~{N}-[(2~{R},3~{R},4~{R},5~{S},6~{R})-5-[(2~{S},3~{R},4~{S},5~{S},6~{R})-4-[[1-[[3-(3-azanylprop-1-ynyl)phenyl]methyl]-1,2,3-triazol-4-yl]methoxy]-6-(hydroxymethyl)-3,5-bis(oxidanyl)oxan-2-yl]oxy-6-(hydroxymethyl)-4-oxidanyl-2-propoxy-oxan-3-yl]ethanamide 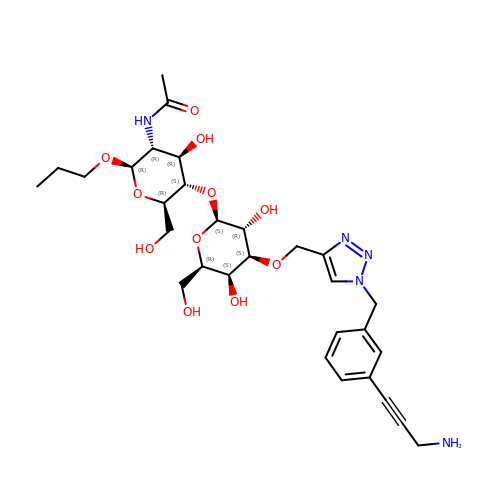| C30 H43 N5 O11 | UZRLHTZEARMTAQ-JSXKIBNASA-N>MVVIDLLIVEVVLFIAALLFSGFFSSSEVALISITRAKVHALQSQGRKGAKALDTLKRSTDAIQITTLIGSTIANVAVASLATAIGITLYGNLGIAVGLVVAAVLVLVFGEIGPKMYASRYTEELALRVSRPILFFSKLLYPVLWVTDRIEQQFAFRPGVTEPVVTEEEIKEWIDVGEEEGTIEEEERDMLYSVLRFGDTTAREVMTPRVDVVMIEDTATLESALAIFNETGFSLIPVYHERIDNIVGLLNVKDVFSAVFRQQTSATIRDLMYEPYFIPESKKIDELLKELQVKKQHMAVVLDEYGSFAGIVTVEDMLEELVHHHHHH[2x]

CNNM/CorB proteins are a broadly conserved family of integral membrane proteins with close to 90,000 protein sequences known. Structurally, CNNM/CorB proteins are defined by a conserved core consisting of a transmembrane domain (TMD) and a cytosolic cystathionine-β-synthase (CBS)-pair domain. Here, we determine the crystal structure of an archaeal CorB ortholog in two distinct conformations (apo and Mg2+-ATP-bound).

Further insight into the conformation in the absence of bound ATP came from the crystal structure of a MtCorBΔC R235L mutant, homologous to a Jalili syndrome mutant (R407L) that is unable to bind ATP in human CNNM4. Crystals of MtCorBΔC R235L mutant purified in UDM were obtained by vapor diffusion in presence of 0.1 M sodium citrate pH 5.5, 50 mM Li2SO4, and 11% PEG4000, but they diffracted poorly to 6 Å. Subsequent additives screening improved the resolution to 3.8 Å with the addition of 10 mM MgSO4. In the apo structure, the TMD remains in the same inward-facing conformation, but the cytosolic domains undergo major structural rearrangements. The CBS-pair domain has completely dissociated from the disc-like dimeric configuration to a more elongated, open conformation with different domain-domain contacts. To our knowledge, this dimeric configuration is not observed in any available CBS-pair domain structures. In agreement with the AUC results, the loss of ATP binding disrupted the dimerization of the CBS-pair domain, which then makes contact with the helix-turn-helix motif from TMD. In addition, the dimeric AHB dissociates and binds to the CBS2 motif of the neighboring molecule, competing for the Mg2+-ATP binding site. The two conformations are interchangeable by a 90° rotation of both protomers. Despite the large dimeric rearrangement, the individual protomer in the two states is similar with differences limited to the AHB and α8 helix.N-methyl-4-{[2-(methylsulfonyl)phenyl]amino}-6-[(pyridin-2-yl)amino]pyridazine-3-carboxamide 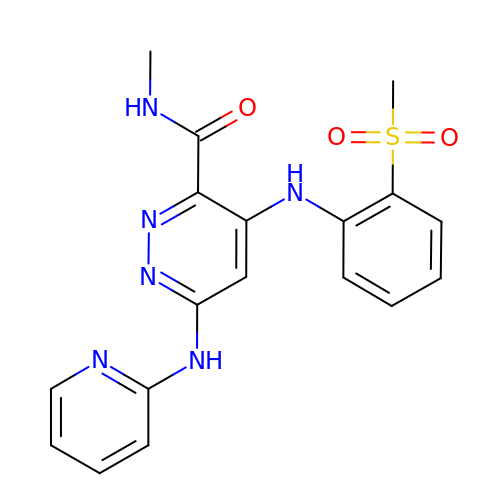| C18 H18 N6 O3 S | KUHISBZXQSKCLH-UHFFFAOYSA-N>[4x]MAVPETRP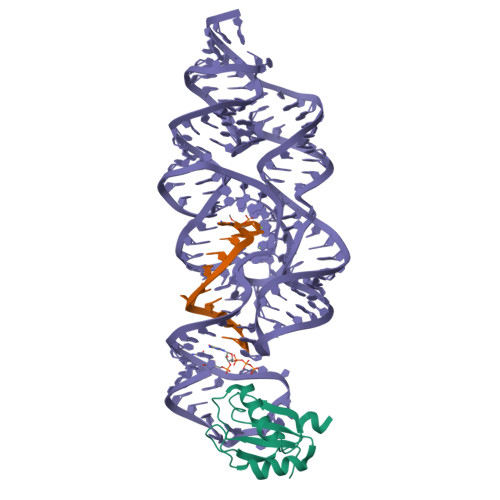NHTIYINNLNEKIKKDELKKSLHAIFSRFGQILDILVSRSLKMRGQAFVIFKEVSSATNALRSMQGFPFYDKPMRIQYAKTDSDIIAKMK> MGSSHHHHHHSSGLVPAGSHMAGTKKGVSAAAFSGVTAALGDVGARWFYTWAADPQGITAPAGTEFVPMIWGRDSVTADQLQRAKAAGSTLLAFNEPDLAGQANMSVETALDLWPQLQATGMRLGAPAVAYGGDTPGGWLDRFMSGAAARGYRVDFIPLHWYGGDFSAAATGQLQSYLQAVYNRYHRPIWLTEYALTDFSGSTPRYPSAAEQADFVSRSTAMLNGLSFVE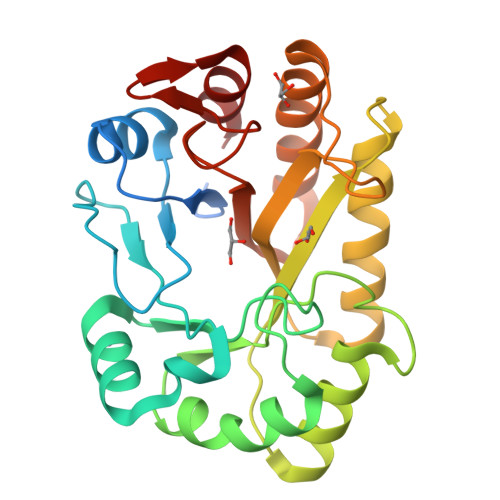RYAWFSLSTSTTPTGLYTGTTPNSSGVAYRAAG> GPGSSEHKAKYENVTKDIFDLRDYYSGASKELKNVTGYRYSKGGKHYLIFDKHQKFTRIQIFGKDIERLKTRKNPGLDIFVVKEAENRNGTVFSYGGVTKKNQGAYYDYLNAPKFVIKKEVDAGVYTHVKRHYIY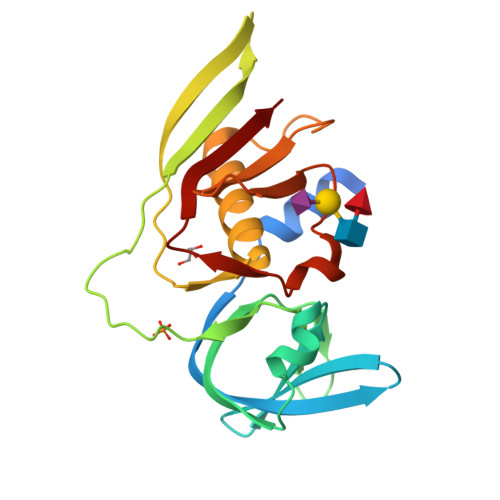KEEVSLKELDFKLRQYLIQNFDLYKKFPKDSKIKVIMKDGGYYTFELNKKLQPHRMSDVIDGRNIEKMEANIR> C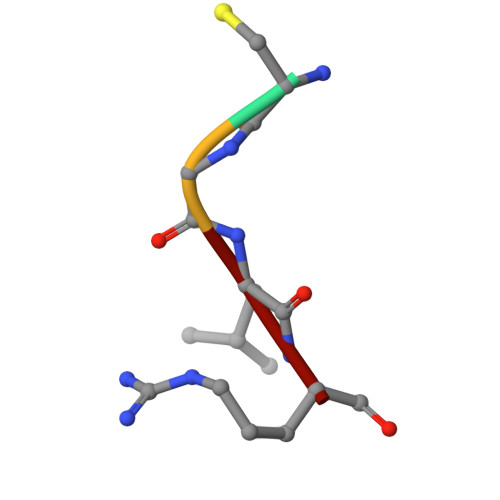GLR>GITGTWYNQLGSTFIVTAGADGALTGTYESAVGNAESRYVLTGRYDSAPATDGSGTALGWTVAWKNNYRNAHSATTWSGQYVGGAEARINTQWLLTSGTTEANAWKSTLVGHDTFTKVKP[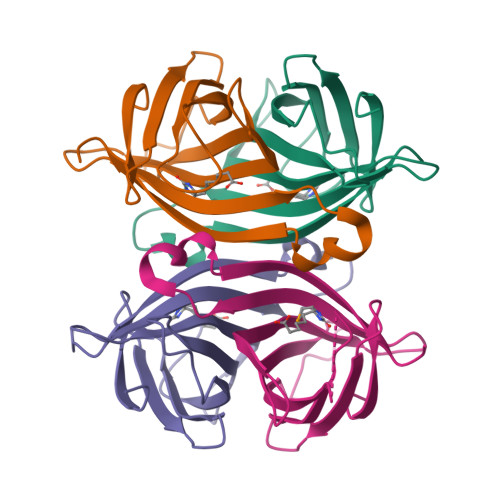4x]1-(1-methylethyl)-3-(naphthalen-1-ylmethyl)-1H-pyrazolo[3,4-d]pyrimidin-4-amine 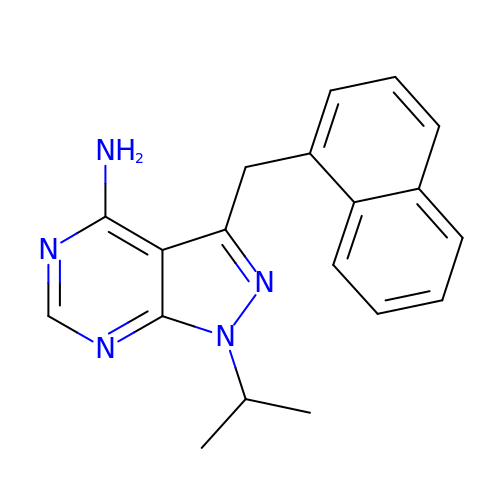| C19 H19 N5 | QFGDRGRJMYSRIW-UHFFFAOYSA-N> GHMTVEYTASDLATYQNEVNEQIAKNKAHLESLTHPGSKVTFPIDQDISATPQNPNLKVFFFDIDNCLYKSSTRIHDLMQQSILRFFQTHLKLSPEDAHVLNNSYYKEYGLAIRGLVMFHKVNALEYNRLVDDSLPLQDILKPDIPLRNMLLRLRQSGKIDKLWLFTNAYKNHAIRCLRLLGIADLFDGLTYCDYSRTDTLVCKPHVKAFEKAMKESGLARYENAYFIDDSGKNIETGIKLGMKTCIHLVENEVNEILGQT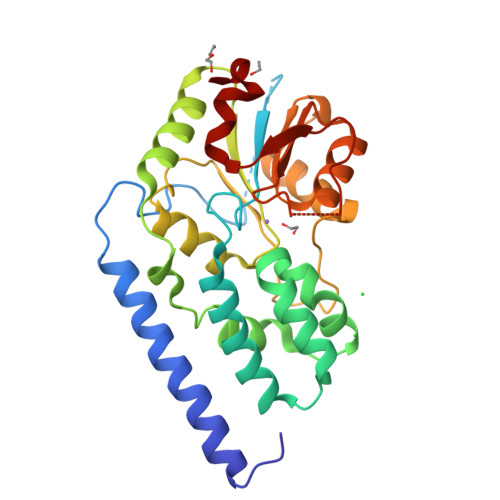PEGAIVISDILELPHVVSDLF NOD2, also known as NLRC2 or CARD15, belongs to the NLRC subfamily of NLRs. NOD2 possesses two tandem CARDs that function as an effector domain and is activated by muramyl dipeptide (MDP), a bacterial cell wall fragment9101112. On activation by MDP, NOD2 is believed to undergo self-oligomerization via the central NOD domain, providing a scaffold for recruiting RIPK2 (receptor-interacting serine–threonine kinase 2) through CARD–CARD interactions. Here, we determined the crystal structure of the inactive ADP-bound form of NOD2, and revealed that ADP-bound NOD2 is maintained in an auto-inhibited/closed form through ADP-mediated and inner domain interactions of the NOD domain.

We also generated a construct in which we deleted the loop regions encoded in residues 245–251 and 626–635, in addition to the removal of the CARD (OcNOD2ΔCARDΔloop), because residues 245–251 are not conserved in zebrafish NOD2 and residues 626–635 are susceptible to proteolytic cleavage during purification. The OcNOD2Δloop construct exhibited activity comparable to the wild-type OcNOD2 in response to MDP, while the OcNOD2SER construct exhibited no activity in NF-κB reporter assays in HEK293T cells. We crystallized OcNOD2ΔCARDΔloop in two forms (form 1 and form 2) under different crystallization conditions and determined the crystal structures at 2.3 Å (form 1) and 3.3 Å (form 2) resolutions. The asymmetric unit of the form 1 and form 2 crystals contained one and two NOD2 molecules, respectively. The structures of the NOD2 molecules in these crystals were essentially the same, with root mean squared deviations (r.m.s.d.) between 0.4 and 1.1 Å. In the crystal structure, the electron density of the ADP molecule was observed clearly, even though it was not supplemented during purification and crystallization. ADP embedded at the centre of the NOD domain bridged the NBD and HD1, and bound to the WHD, allowing the subdomains to be closely packed.

> GPEFEAAACKKYMSKLRTIVAAQSRFLSTYDGAENLCLEDIYTENTLEVRTEVGMAGPLHKSPAALGLEELFSPNGHLNEDADTVLVVGEAGSGKSTLLQQVHLLWATGQDFQEFLFVFPFSCRQLQCVARPLSVMTLLFEHCCWPDVGQQDVFQFLLDHPDRILLTFDGFDEFKFKFTDHERHCSPTDPTSVQTLLFNLLQGNLLKNARKVLTSRPDAVSAFLRKYVRTEFNLKGFSEEGIELYLRKCHREPGVADRLIHLLQTTSALHGLCHLPVFSWMVSKCHQELLLQDGGSPKTTTDMYLLILQHFLRHASLPDSASQGLGPSLLQGRLPTLLRLGQLALWGLGMCCYVFSAQQLQAAQVDPDDISLGFLVQAQGVVPGSTAPLEFLHITFQCFLAAFYLVLSTDVPTASLRYLFNCRRPGSSPLSRLLPRLCVQGSEHKESTVAALLQKTEPHNLQITAAFLAGLLSREHRDLLAACQASERSLLRRRACARWCLARSLHKHFRSIPPAVPGEAKSMHAMPGFLWLIRSLYEMQEERLAQEAVRGLNVEHLKLTFCGVGPAECAALAFVLRHLRRPVALQLDHNSVGDIGVEQLLPCLGACKALYLRDNNISDRGICKLIEHALHCEQLQKLALFNNKLTDGCAHSVAQLLACKQNFLALRLGNNHITAEGAQVLAEGLRDNSSLQFLGFWGNKVGDKGAQALAEALSDHQSLKWLSLVGNNIGSVGAQALASMLEKNVALEELCLEENHLQDAGVCSLAEGLKRNSSLKVLKLSNNCITFVGAEALLQALASNDTILEVWLRGNPFSPEEMEALSHRDSRLLL> CQDPTIFEERHLKYISQLGK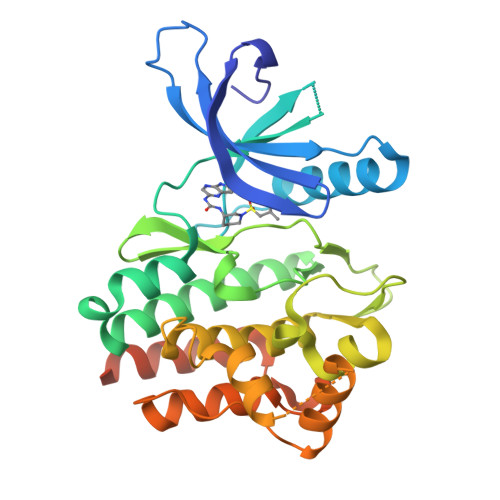GNFGSVELCRYDPLGDNTGALVAVKQLQHSGPDQQRDFQREIQILKALHSDFIVKYRGVSYGPGRQSLRLVMEYLPSGCLRDFLQRHRARLDASRLLLYSSQICKGMEYLGSRRCVHRDLAARNILVESEAHVKIADFGLAKLLPLDKDYYVVREPGQSPIFWYAPESLSDNIFSRQSDVWSFGVVLYELFTYCDKSCSPSAEFLRMMGSERDVPALSRLLELLEEGQRLPAPPACPAEVHELMKLCWAPSPQDRPSFSALGPQLDMLWSGSRGCETHAFTAHPEGKHHSLSFS~{N}-[(5-azanyl-1,3,4-oxadiazol-2-yl)methyl]-2-(2-chlorophenyl)sulfanyl-~{N}-[(4-cyanophenyl)methyl]ethanamide 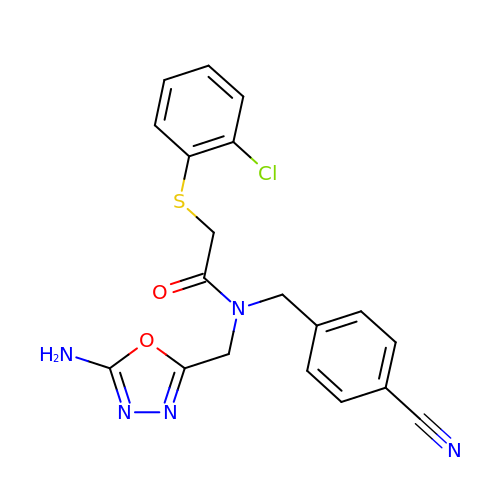| C19 H16 Cl N5 O2 S | DDHNQWBEECYOFY-UHFFFAOYSA-N>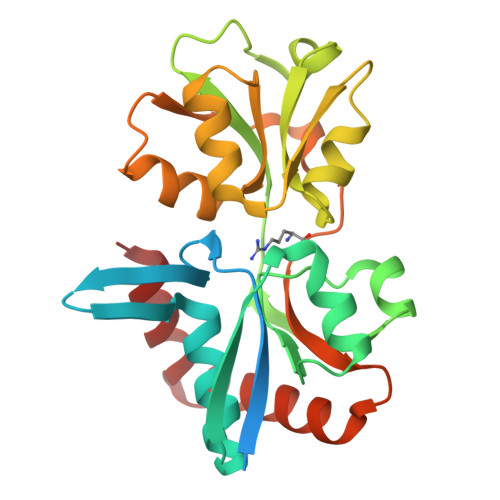MNKKSLFLAFAVVFALAFMLSGCGSKFNTVDQIKQKGVIVMGTSADFPPFEFHKVEGGKDEIVGFDIDIANAIAKKLGVKLEIKDMDFKGLIPALQAGRVDMVIAGMTPTAERKKSVDFSDLYYDSRQVVVVKNDSPISKFDDLKVKTIAVQIGTTSEEAAKKIPNVKLKQLNRVSDEFMDLQNGRCDAIVVEDTVAKAYLKEYKDMKILYMDEINNVENGSAVAVAKGNKSLLDVVNEVIKELKQSGEYDKLVDKWFKQ[2x]>GSHMLEFSEWYSDILEKAEIYDVRYPIKGCGVYLPYGFKIRRYTFEIIRNLLDESGHDEALFPMLIPEDLLAKEAEHIKGFEDEVYWVTHGGKTQLDVKLALRPTSETPIYYMMKLWVKVHTDLPIKIYQIVNTFRYETKHTRPLIRLREIMTFKEAHTAHSTKEEAENQVKEAISIYKKFFDTLGIPYLISKRPEWDKFPGAEYTMAFDTIFPDGRTMQIATVHNLGQNFSKTFEIIFETPTGDKDYAYQTCYGISDRVIASIIAIHGDEKGLILPPIV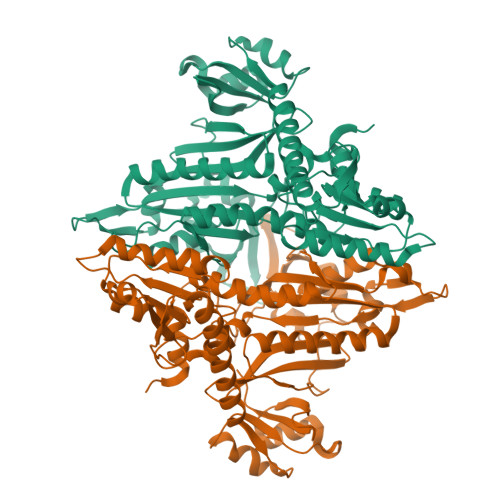APIQVVIVPLIFKGKEDIVMEKAKEIYEKLKGKFRVHIDDRDIRPGRKFNDWEIKGVPLRIEVGPKDIENKKITLFRRDTMEKFQVDETQLMEVVEKTLNNIMENIKNRAWEKFENFITILEDINPDEIKNILSEKRGVILVPFKEEIYNEELEEKVEATILGETEYKGNKYIAIAKTY[4x]>[2x]MADPESPWSQIGRKIKLEGLSDVASISTKLQNTLIQYHSIEEDEWRVAKKAKDVTVWRKPSEEFNGYLYKAQGVMDDVVNNVIDHIRPGPWRLDWDRLMTSLD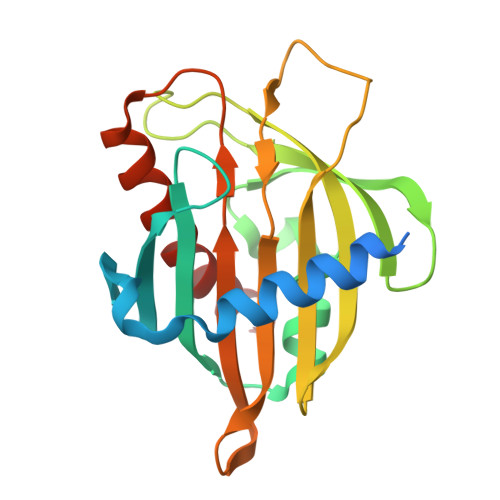VLEHFEENCCVMRYTTAGQLLNIISPREFVDFSYTVGYEEGLLSCGVSVEWSETRPEFVRGYNHPCGWFCVPLKDSPSQSLLTGYIQTDLRGMIPQSAVDTAMASTLANFYSDLRKGLRKA> MEPAGRFTKVAAAVADSVVTIESVSDQEGMQGSGVIVDGRGYIVTNAHVISEAANNPSQFKTTVVFNDGKEVPANLVGR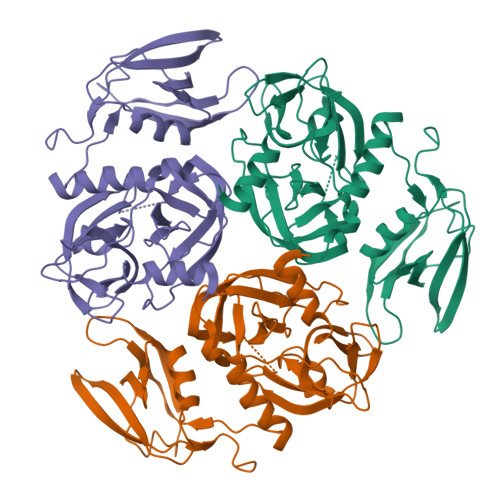DPKTDLAVLKVDNVDNLTVARLGDSSKVRVGDEVLAVGAPLGLRSTVTQGIVSALHRPVPLSGEGSDTDTVIDAIQTDASINHGNSGGPLIDMDAQVIGINTAGKSLSDSASGLGFAIPVNEMKLVANSLIKDGKIVHPTLGISTRSVSNAIASGAQVANVKAGSPAQKGGILENDVIVKVGNRAVADSDEFVVAVRQLAIGQDAPIEVVREGRHVTLTVKPDPDSTLEHHHHHH> GHMGEIRPTIGQQMETGDQRFGDPVFRQL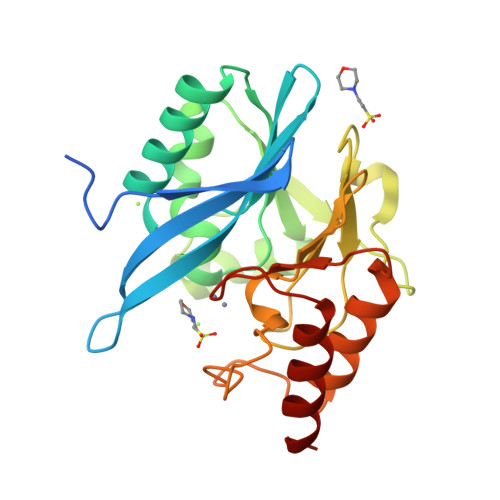APNVWQHTSYLDMPGFGAVASNGLIVRDGGRVLMVDTAGTDAQTAQILKWIKQEINLPVALAVVTHAHQDKMGGMDALHAAGIATYANALSNQLAPREGVVAAQHSLTFAATGWVEPATAPNFGPLKVFYPGPGHTSDNITVGIDGTDIAFGGCLIRDSKAKSLGNLDEADTEHYAASVRAFGAAFPKASMIVMSHFAPDSRAAITHTARMADKLR> GPSQVIFNSVE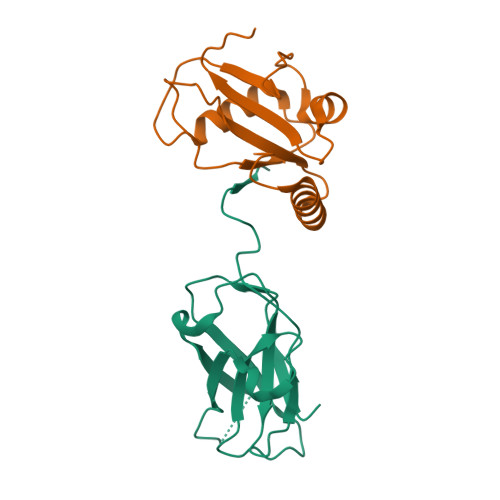KFYIPGGDVTCHYTFTQHFIPRRKDWIGIFRVGWKTTREYYTFMWVTLPIDLNNKSAKQQEVQFKAYYLPKDDEYYQFCYVDEDGVVRGASIPFQFRPENEEDILVVTTQGE;> GPMPPPQKIPSVRPFKQRKSLAIRQEEVAGIRAKFPNKIPVVVERYPRETFLPPLDKTKFLVPQELTMTQFLSIIRSRMVLRATEAFYLLVNNKSLVSMSATMAEIYRDYKDEDGFVYMTYASQETFG>MERLDIFGVPIDRVTMIQAVDILNNFLQENRLHIVATPNAEIVMMAQKDKEYMEILNNTDLNVPDGSGIVFASKVFKKPLPERVAGFDLMLEFIKGISSKGVKIYLLGAAAQVAEQARANLEKLYPGVKIVGTHHGYFTEEEENKIIEEINNKGAEVLFVALGAPKQEKWIYKNKDKLKVKIAMGVGGSFDVIAG[8x]

The TagA N-acetylmannosamine transferase catalyzes the first committed step in WTA biosynthesis. The TagA glycosyltransferase (GT) then appends ManNAc from a UDP-ManNAc donor, producing a C55-PP-GlcNAc-ManNAc disaccharide-lipid product (lipid-β). To gain insight into the mechanism of catalysis, we determined the 2.0 Å crystal structure of the TagA enzyme from Thermoanaerobacter italicus (TagAΔC, residues Met1-Gly195). TagAΔC contains the highly conserved amino acid region that defines the WecB/TagA/CpsF family, but lacks 49 C-terminal residues that target the protein to the membrane (see below).

Selenomethionine (SeMet)-labeled TagAΔC in its apo-form crystallized in the P21 space group as a dimer, with eight molecules per asymmetric unit. The subunits in the dimer are related by two-fold non-crystallographic symmetry and possess similar atomic structures; their heavy atom coordinates can be superimposed with an RMSD of 0.11 Å. Each protomer consists of eight β–strands and nine α-helices that form two distinct regions. The N-terminal region of TagA is formed by helices H2 to H4 that pack against a β-hairpin constructed from strands β1 and β2, while its larger C-terminal region is comprised of a six-stranded parallel β-sheet (β–strands β4, β3, β8, β7, β5, and β6) that is surrounded by seven helices (helices H1, H3, and H5 to H9). The arrangement of the six parallel strands forming the β–sheet resembles a Rossmann fold commonly found in nucleotide-binding proteins. In the dimer, the C-terminal helix H8 in one subunit packs against helices H2 and H4 located in the N-terminal region of the adjacent protomer, burying 1,212 Å2 of solvent accessible surface area to produce a narrow pore (detailed in S6 Fig). Analytical ultracentrifugation (AUC) experiments indicate that TagAΔC dimerizes in solution with relatively weak affinity, with a monomer-dimer dissociation constant (Kd) of only 7.4 ± 0.7 μM. Consistent with the native and SeMet-labeled proteins adopting similar quaternary structures, introduction of V43E and A72R mutations into TagAΔC disrupts dimerization. The C-terminal appendage is presumably unstructured in dimeric forms of the enzyme, as, importantly, the contact surface used to engage the appendage is occluded by inter-subunit interactions in the crystal structures of TagAΔC.> EMKVAVITGASRGIGEAIARALARDGYALALGARSVDRLEKI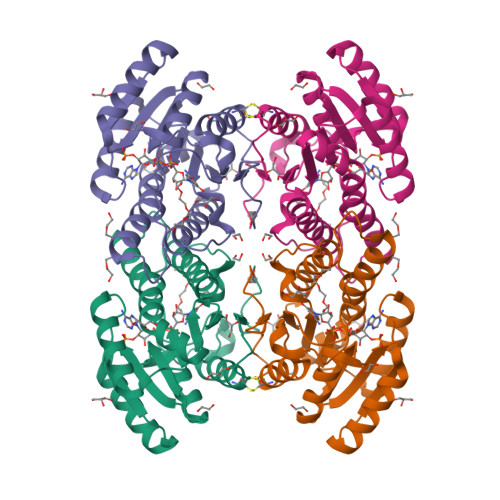AHELMQEQGVEVFYHHLDVSKAESVEEFSKKVLERFGDVDVVVANAGLGYFKRLEELSEEEFHEMIEVNLLGVWRTLKAFLDSLKRTGGLALVTTSDVSARLIPYGGGYVSTKWAARALVRTFQIENPDVRFFELRPGAVDTYFGGSKPGKPKEKGYLKPDEIAEAVRCLLKLPKDVRVEELMLRSVYQRPEY>[6x]SLTEIEHLVQSVCKSYRETCQLRLEDLLRQRSNIFSREEVTGYQRKSMWEMWERCAHHLTEAIQYVVEFAKRLSGFMELCQNDQIVLLKAGAMEVVLVRMCRAYNADNRTVFFEGKY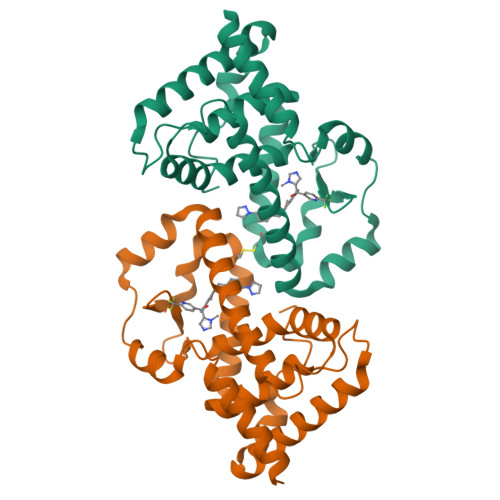GGMELFRALGCSELISSIFDFSHSLSALHFSEDEIALYTALVLINAHRPGLQEKRKVEQLQYNLELAFHHHLHKTHRQSILAKLPPKGKLRSL> MGKKELKRGLVVDREAQMIGVYLFEDGKTYRGIPRGKVLKKTKIYAGDYVWGEVVDPNTFAIEEVEERKNLLIRPKVA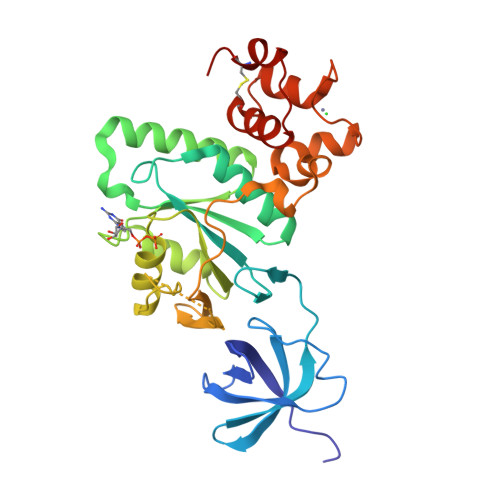NVDRVIIVETLKMPEFNNYLLDNMLVVYEYFKVEPVIVFNKIDLLNEEEKKELERWISIYRDAGYDVLKVSAKTGEGIDELVDYLEGFICILAGPSGVGKSSILSRLTGEELRTQEVSEKTERGRHTTTGVRLIPFGKGSFVGDTPGFSKVEATMFVKPREVRNYFREFLRYQCKYPDCTHTNEPGCAVKEAVKNGEISCERYKSYLKIIKVYLEEIKELCRED GDP-ALPHA-D-GLUCOSE | C16 H25 N5 O16 P2 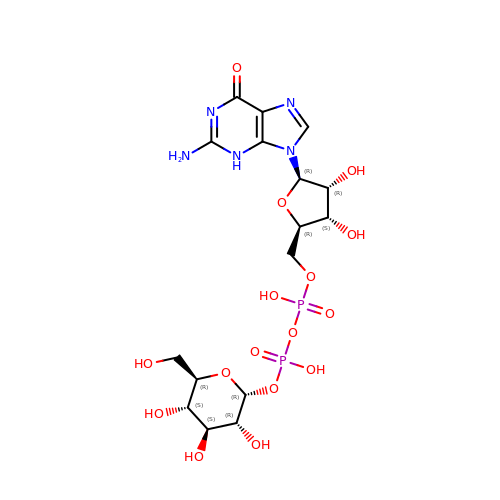| MVMSCBBUIHUTGJ-LRJDVEEWSA-N> MAMANNSSVANKVCLIVIDGWGVSEDPYGNAILNAQTPVMDKLCSGNWAQIEAHGLHVGLPEGLMGNSEVGHLNIGAGRVIYQDIVRINLAVKNNKFVTNESLVDACDRAKNGNGRLHLAGLVSDGGVHSHIDHMFALVKAIKELGVPELYLHFYGDGRDTSPNSGVGFLEQTLEFLEKTTGYGKLATVVGRYYAMDRDNRWERINVAYEAMIGGVGETSDEAGVVEVVRKRYAADETDEFLKPIILQGEKGRVQNDDTIIFFDYRADRMREISAAMGMDRYKDCNSKLAHPSNLQVYGMTQYKAEFPFKSLFPPASNKNVLAEWLAEQKVSQFHCAETEKYAHVTFFFNGGLEKQFEGEERCLVPSPKVATYDLQPEMSAA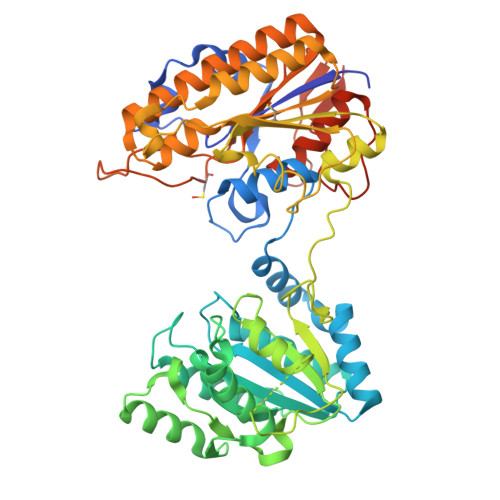GVADKMIEQLEAGTHPFIMCNFAPPDMVGHTGVYEAAVKACEATDIAIGRIYEATQKHGYSLMVTADHGNAEKMKAPDGGKHTAHTCYRVPLTLSHPGFKFVDPADRHPALCDVAPTVLAIMGLPQPAEMTGVSIVQKIKLAAALEHHHHHHHHHH>GSFTEELHLIPPLNFSMVDNGIFRSGFPDSANFSFLQTLGLRSIIYLCPEPYPESNLQFLKSNGIRLFQFGIEGNKEPFVNIPDHKIRMALKVLLDEKNHPVLIHSKRGKHRTGCLVGCLRKLQKWCLTSIFDEYQRFAAAKARVSDQRFMEIFDVSSFSHIPMSFSCSIR[2x]

Here, we provide the ligand/enzyme crystal complexes for one such PTP outlier: Arabidopsis thaliana Plant and Fungi Atypical Dual Specificity Phosphatase 1 (AtPFA-DSP1), herein unveiled as a regioselective and efficient phosphatase towards inositol pyrophosphate (PP-InsP) signaling molecules. Although the WPD loop is missing its canonical tripeptide motif, this structural element contributes to catalysis by assisting PP-InsP delivery into the catalytic pocket, for a choreographed exchange with phosphate reaction product. Subsequently, an intramolecular proton donation by PP-InsP substrate is posited to substitute functionally for the absent aspartate/glutamate general-acid. Additionally, we conclude that the hydrolyzed phosphate remains trapped as an enzyme-product complex, until it can be released in a prisoner exchange with another PP-InsP molecule; the latter process is assisted by the WPD loop.

The oxygen atom that is positioned at the apex of the phosphate ion’s tetrahedral geometry points away from α4. This oxygen makes a hydrogen bond with the unprotonated Nδ1 of His155 (we will return to this point below). We denote this orientation of Pi as pose A, i.e., Pi(A). The three other oxygen atoms of this Pi are intensively coordinated by amide groups of P-loop residues Lys151, Arg152 Lys154, His155, and Arg156. The side chains of Arg156 and Cys150/Ser150 also make polar contacts with Pi(A).> MAEEANKDADISSLSLSLDPEIIGGQNNFLENNLQQIFQKIIQERGPFRDLKEEDLQKELQKESIKDESSAKSSETENVLEFATLDSKRNVNDTEVESMDSQAYK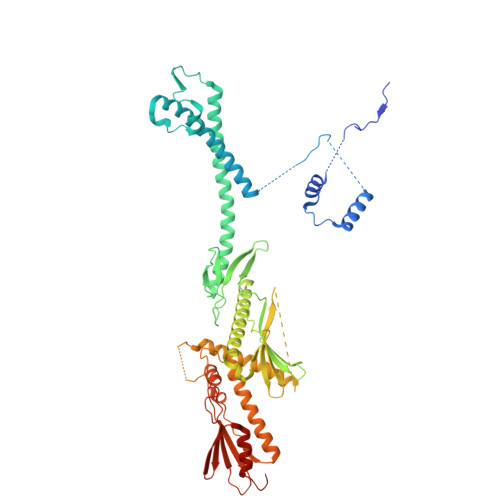KELIEQIMIAQTECSLALDMTSLLLSKFKENSIETISPFLKSTVPPSSLQFSRSQPPESKESDATLAKCWKEKSLTSSCKFLFEAKERLTSVVETEHEYYTELVKVKEASWPLFNSQGSNHLSVQYSCLGGISLGLGLIRMKPESKSFEVQSSLLYSQAALKISILNKDRDEIGSSTWSWPSQNCNSVLLKDIYKLQEILFEMDIWNSLLQEAQSCGNQGVNFTGDEILVPISDDHVVRITLETSSKNTESGFTEDKKSNEDTSTNFVTIKQEKELLKCLCDTLNAIAHILFLKHCRKSDRRSQQPELYMAIDANAPLILRPLIFYYNLNQESLEFQRWLKQRDISFKFMPNYPWEKAKDFLELENSLSINRLSISWRIMVSNFEPAIFIQHTPTLHGTDKSVWRCKDQYSSNQFSSLKNVCQYIEHHINSLSRRSKKTE> SMDMPVERILEAELAVEPKTETYVEANMGLNPSSPNDPVTNICQAADKQLFTLVEWAKRIPHFSELPLDDQVILLRAGWNELLIASFSHRSIAVKDGILLATGLHV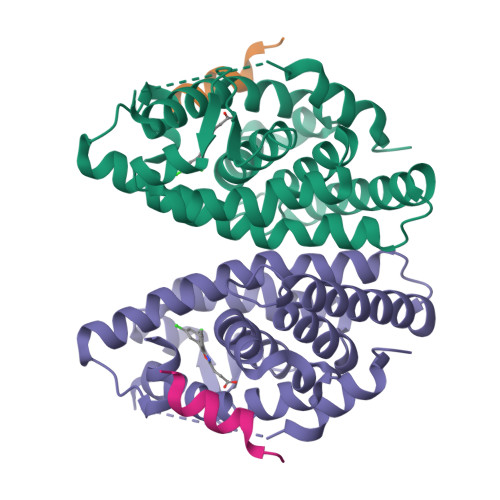HRNSAHSAGVGAIFDRVLTELVSKMRDMQMDKTELGCLRAIVLFNPDSKGLSNPAEVEALREKVYASLEAYCKHKYPEQPGRFAKLLLRLPALRSIGLKCLEHLFFFKLIGDTPIDTFLMEMLE;> KHKILHRLLQDSSY> MSILNDYKRKTEGSVFWAQRARSVMPDGVTADTRVFDPHGLFISDAQGVHKTDVDGNVYLDFFGGHGALVLGHGHPRVNAAIAEALSHGVQYAASHPLEVRWAERIVAAFPSIRKLRFTGSGTETTLLALRVARAFTGRRMILRIATHYHGWHDFSASGYNSHFDGQPAPGVLPEIAKNTLLIRPDDIEGMREVFAQHGSDIAA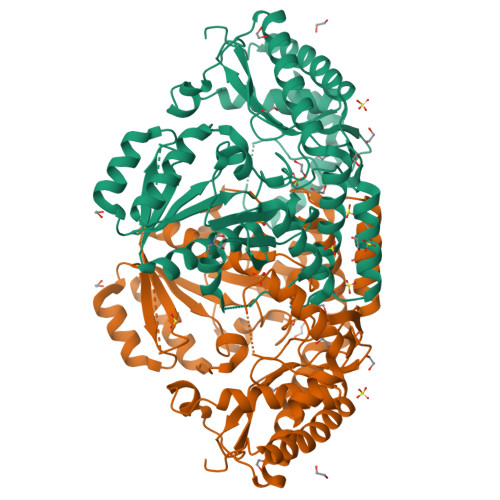FIAEPVGSHFGVTPVSDSFLREGAELARQYGALFILDEVISGFRVGNHGMQALLDVQPDLTCLAKASAGGLPGGILGGREDVMGVLSRGSDRKVLHQGTFTGNPITAAAAIAAIDTILEDDVCAKINDLGQFAREAMNHLFARKGLNWLAYGRFSGFHLMPGLPPNTTDTGSITRAEVARPDVKMIAAMRMALILEGVDIGGRGSVFLSAQHEREHVEHLVTTFDRVLDRLADENLLSWQPTNLSGNQS> GSSQLPQNIQFSPSAKLQEVL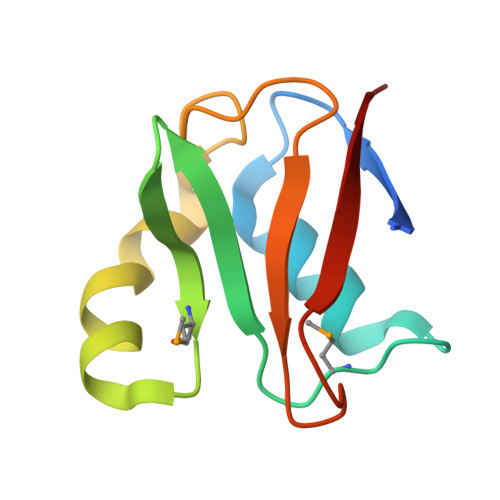DYLTNSASLQMKSPAITATLEGKNRTLYMQSVTSIEERTRPNLSKTLKELGLVDGQELAVADVTTPQTVLFKLHFTS>[6x]MKIYRPLWEDGAFLMPQQFQQQAAWDVHLADSVARMGLAHPWGVVAAEFDDSLLPLSRLNATRLIVRFPDGTLIDTERADNLPPVCDLSTVSDRSLVDIVLALPLLNANGGNLDNGSESERPRRWKSERVNVQELAGHEQSEVAVLRHNLTLRMAHQENAAWLTCPVTRLVRDAQGQWCRDPRFIPPLLTLSASPSLMTELAELLHHLQARRQRLMSMRRENNARLADFAVADVSLFWLLNALNSAEPVLKELLDMPYRHPELLYRELARLAGSLLTFSLEHNVDAVPAYHHETPENVFPPLLSLLNRLLEASLPSHHHHHH;> MGFPASEIKDAVIPEESHLPPIVHVTFMGLYGVTSPLPAHYISDIAQQREGHEAAADFLDIFSHRLITQYYRIWRKYSYPATFEAGGQDKTSQYLLGLARLGIPGCAQNIATPVSRFLALLPLMLLPGRTAEGLTSLVTLLAPGTQARVWHHDRRRIPLKTPLTMRVHHPVSLKSRPVMGDHATDVNGQVLLQLSTQTGSEVQGWLPGGHLYSDLLALLHVYLGSRLDVRLQLCVERSLLPDARLSCRPAAGSPQLGRTAVMRTQAKIATSAARVMTISLGRYQRVQEHYQRKETQENGDYRW;>[2x]MDDLTLRYFDAEMRYLREAGKAFAQAHPDRAAMLDLDKAGTPDPCVERLFEGFAFSMGRLRQKIDDDLPELTESLVSMLWPHYLRTIPSLSVVALTPRLSVMKMAETVPAGLEVTSRPVGPGNTVC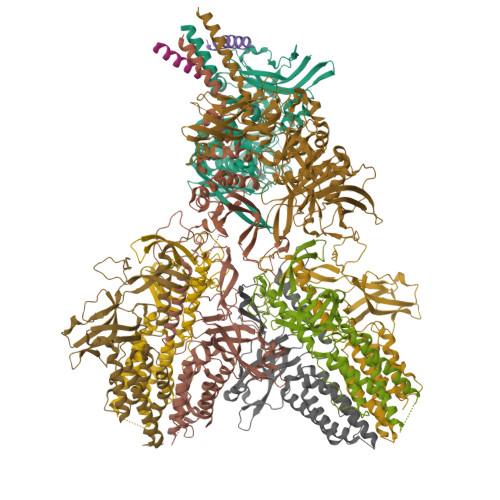RYRTTRAIPLNPLAVEKVVMTTEPDGRSVLKIGFACSELADWSQVDLHRLSLYLAAEAPVSSTLHLMMTKRLAALYLRLPGNDERIRIDGWFSPGGFAEEDRLWPKGDSAFSGYQLLLEYFTFREKFMFVHLNGLENVSLPAGISGFDLEVVLSQPWPADLPVTDDALCLHCVPVINLFTLEADPLIINGLESEYLLRPKRLQDGYTEIYSVDAVTGSGRTGSAEYVPFTSFRHRGGMLRHDAPERYYHTRVKRGVTGMYDTWLILGGQRWEADRMPERETLSLRITGTNGQLPRRALQSTLLDRCEQVLQAPVSVRNLCKPTLPVYPPTEDRFHWRVMSHLGTGFLNMLSSAEVLRGTLALYNWRDDELNHRRLDAILAVQHHRIQRFEKGFLLRGLDVEVTLDGNGFAGEGDIHLFGEMLNRFLALYADMNQFNQLTLIVQPEGKCIRWKENHNPRLPG Dipeptidyl peptidase-4 (DPP-4), the serine protease responsible for metabolism of the incretin hormones glucagon-like peptide-1 and glucose-dependent insulinotropic polypeptide, plays an important role in regulating glucose homeostasis. Thus, DPP-4 is an attractive target for therapeutic intervention, and inhibitors of DPP-4 have been shown to be an effective therapy for treatment of T2DM. Trelagliptin (SYR-472, zafatek) is a novel once-weekly DPP-4 inhibitor approved in Japan.

The 2-position carbonyl participates in an important hydrogen bond with the backbone NH of Tyr631, and the uracil ring π-stacks with Tyr547. The single chemical structural difference between the two compounds is the presence of a fluorine atom at the 5-position of the cyanobenzyl group. Examination of the environment around the fluorine atom in the DPP-4 active site reveals the proximity of residues Trp659, Tyr631, and Val656. Of these residues, only hydrogen atoms are within Van der Waals distance of the fluorine. These hydrogen atoms carry a permanent partial positive charge due to the position on the aromatic rings of Trp659 and Tyr631, and an inducible positive charge on the side chain of Val656. Fluorine carries a permanent partial negative change and so these atoms would be expected to produce an additional attractive force between ligand and protein, compared to a hydrogen atom at the 5-position. The magnitude of this attraction would be expected to be small but may be responsible for the 4-fold potency increase observed for trelagliptin versus alogliptin. X-ray diffraction data confirms that trelagliptin binds to DPP-4 in a pose that is virtually identical to that seen for alogliptin, with the exception of the single fluorine atom at the 5-position of the cyanobenzyl group which may account for the slight potency advantage for trelagliptin.

>ADPGGSHHHHHHSRKTYTLTDYLKNTYRLKLYSLRWISDHEYLYKQENNILVFNAEYGNSSVFLENSTFDEFGHSINDYSISPDGQFILLEYNYVKQWRHSYTASYDIYDLNKRQLITEERIPNNTQWVTWSPVGHKLAYVWNNDIYVKIEPNLPSYRITWTGKEDIIYNGITDWVYEEEVFSAYSALWWSPNGTFLAYAQFNDTEVPLIEYSFYSDESLQYPKTVRVPYPKAGAVNPTVKFFVVNTDSLSSVTNATSIQITAPASMLIGDHYLCDVTWATQERISLQWLRRIQNYSVMDICDYDESSGRWNCLVARQHIEMSTTGWVGRFRPSEPHFTLDGNSFYKIISNEEGYRHICYFQIDKKDCTFITKGTWEVIGIEALTSDYLYYISNEYKGMPGGRNLYKIQLSDYTKVTCLSCELNPERCQYYSVSFSKEAKYYQLRCSGPGLPLYTLHSSVNDKGLRVLEDNSALDKMLQNVQMPSKKLDFIILNETKFWYQMILPPHFDKSKKYPLLLDVYAGPCSQKADTVFRLNWATYLASTENIIVASFDGRGSGYQGDKIMHAINRRLGTFEVEDQIEAARQFSKMGFVDNKRIAIWGWSYGGYVTSMVLGSGSGVFKCGIAVAPVSRWEYYDSVYTERYMGLPTPEDNLDHYRNSTVMSRAENFKQVEYLLIHGTADDNVHFQQSAQISKALVDVGVDFQAMWYTDEDHGIASSTAHQHIYTHMSHFIKQCFSLP[4x]>[2x]GPLGSMELKYNCILNIKYEMDRDKLVDSSGYRSRINIGTGVKFSEIDKNQVQLSNLESSKIEVILNNGVIYNSMYENFSTSFWIRIPKYFRNINNEYKIISCMQNNSGWEVSLNFSNMNSKIIWTLQDTEGIKKTVVFQYTQNINISDYINRWIFVTITNNRLSNSKIYINGRLINEESISDLGNIHASNNIMFKLDGCRDPHRYIWIKYFNLFDKELNKKEIKDLYDNQSNSGILKDFWGDYLQYDKPYYMLNLYDPNKYLDVNNVGIRGYMYLKGPRGRIVTTNIYLNSTLYMGTKFIIKKYASGNKDNIVRNNDRVYINVVVKNKEYRLATNASQAGVEKILSAVEIPDVGNLSQVVVMKSENDQGIRNKCKMNLQDNNGNDIGFIGFHQFNNIAKLVASNWYNRQIGKASRTFGCSWEFIPVDDGWGESSL

BoNTs specifically target neuromuscular junctions (NMJ), where the toxins are internalized into neuronal cells, cleave the soluble N-ethylmaleimide sensitive factor attachment protein receptors (SNAREs) complex, inhibit the release of neurotransmitter acetylcholine, and eventually paralyze the affected muscles. Structurally, BoNT consists of an N-terminal light chain (LC, ~50 kDa) that is a metalloprotease and a C-terminal heavy chain (HC, ~100 kDa). The latter could be further divided into two domains: the N-terminal portion (~50 kDa) is the translocation domain (HN) required for the LC to be released into the cytosol; the C-terminal part (HC) is the receptor-binding domain responsible for the highly specific binding and endocytosis of BoNT into motoneurons. Amino acid (AA) sequence alignments based on genome sequences of strain IBCA10-7060 showed that the HC of this toxin is most similar to that of BoNT/A1 (~84% identity), while its LC and HN share ~81% and ~64% identity to that of BoNT/F5, respectively.

We then determined the crystal structure of HCHA at 1.8 Å resolution. After large-scale crystallization screens, HCHA was successfully crystallized at 1 mg/mL, an unusually low protein concentration for protein crystallization in general. Dramatically different solubility in solution was observed between HCHA and HCA1, which was largely caused by variation of a single residue (HCA1-R1156 and HCHA-M1148). In BoNT/A8, this loop is longer than that in other subtypes because of a unique arginine insertion that makes BoNT/A8 the longest BoNT/A subtype. The third notable difference is that a 3/10-helix (residues S955-S957) linking β8 and β9 in HCA1 is unstructured in HCHA due to the deletion of two residues in this region (Figure 1B, yellow box). In HCHA this loop (residues E1218-K1226) swings ~45 degrees towards the center of the HCC subdomain compared to that of HCA1. This is likely caused by residue HCHA-R1224 (equivalent to HCA1-T1232), which forms multiple hydrogen bonds with residues R1005 and W1006. The alignment also suggests that a surface-exposed loop in the GBS neighborhood on BoNT/HA (residues I1263-A1266) is highly similar to BoNT/A8 (residues V1272-A1275), but differs from BoNT/A1 (residues I1271-S1274) (blue arrows). This region of HCHA is likely flexible because the electron densities from residues R1261-R1268 were missing in our structure. For example, an arginine on HCA1 (R1156) that contributes a crucial cation-π interaction with SV2C-F563 is replaced by a methionine (M1148) on HCHA. Furthermore, while HCA1-R1294 forms three hydrogen bonds with C520, T521, and D539 of SV2C through its long, well-extended side-chain, these hydrogen bondings are likely missing on HCHA because HCA1-R1294 is replaced by a serine (HCHA-S1286).>[4x]MTHHYPTDDIKIKEVKELLPPIAHLYELPISKEASGLVHRTRQEISDLVHGRDKRLLVIIGPCSIHDPKAALEYAERLLKLRKQYENELLIVMRVYFEKPRTTVGWKGLINDPHLDGTFDINFGLRQARSLLLSLNNMGMPASTEFLDMITPQYYADLISWGAIGARTTESQVHRELASGLSCPVGFKNGTDG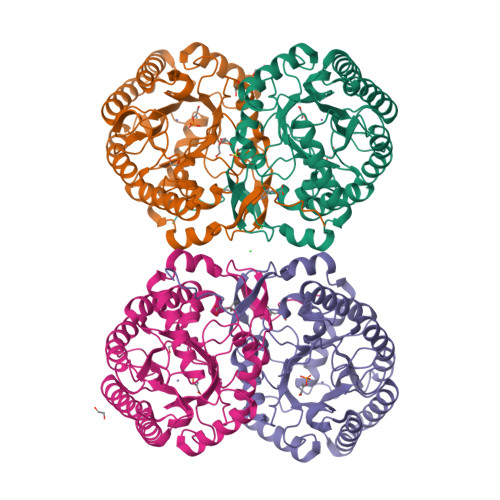NLKIAIDAIGAASHSHHFLSVTKAGHSAIVHTGGNPDCHVILRGGKEPNYDAEHVSEAAEQLRAAGVTDKLMIDCSHANSRKDYTRQMEVAQDIAAQLEQDGGNIMGVMVESHLVEGRQDKPEVYGKSITDACIGWGATEELLALLAGANKKRMARAS>GGGCCNGUCGUCUAXCCUGGUUAGGACGCCGCCCUUACAAGGCGGAGGXCCUGGGUUCGAGUCCCAGCGGGCCCACCA[2x]

Here we identified 2′-phosphouridine (Up) at position 47 of tRNAs from thermophilic archaea. Up47 confers thermal stability and nuclease resistance to tRNAs. In addition, we identified the arkI gene, which encodes an archaeal RNA kinase responsible for Up47 formation. Taken together, our findings show that Up47 is a reversible RNA modification mediated by ArkI and KptA that fine-tunes the structural rigidity of tRNAs under extreme environmental conditions.

To determine the molecular basis for thermal stabilization of tRNA by Up47, we crystalized S. tokodaii tRNAVal3 and determined its atomic structure at a resolution of up to 1.9 Å by X-ray crystallography. One unit cell contains two tRNA molecules, denoted as molecule A and molecule B. Molecule A formed a canonical tRNA core structure, whereas molecule B had an altered core structure with a non-canonical base triple. We clearly observed electron densities for tRNA modifications, including Up47. In both molecules, the 2′-phosphate of Up47 was oriented towards the solvent side and did not interact with any residues. The O4′ position in the ribose of Up47 formed a hydrogen bond with the N6-amino group of A21 in both molecules. The uracil base of Up47 faced the tRNA core. Although molecule A had a canonical tRNA core structure stabilized by multiple tertiary interactions between the D-arm and V-loop, including the base triples s4U8– A14–A21, Ψ13–G22–G46, C12–G23–C9 and m2G10–C25–G45, molecule B unexpectedly had a non-canonical core structure. In molecule B, G46 was dissociated from the base triple Ψ13–G22–G46 and stacked with Up47. To compensate for this conformational change, C9 comes up from the lower layer (C12–G23–C9) to form the non-canonical base triple Ψ13–G22–C9. Up47 catches the G46 base that is dissociated from the base triple to restrict further rotation of the V-loop, thereby stabilizing the metastable core structure of the tRNA to prevent its heat denaturation.4-[2-methyl-1-(4-methylpiperazin-1-yl)-1-oxidanylidene-propan-2-yl]-~{N}-(6-pyridin-4-ylimidazo[1,2-a]pyridin-2-yl)benzamide | C28 H30 N6 O2 | 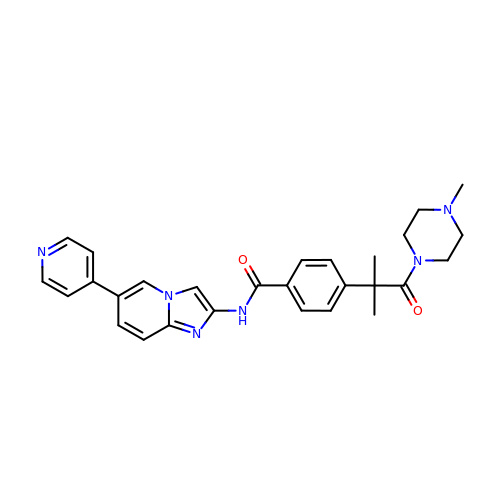IEFFSHLHNYVSEF-UHFFFAOYSA-N4-bromo-2-methyl-5-[[(3~{R},5~{R})-1-methyl-5-phenyl-piperidin-3-yl]amino]pyridazin-3-one | C17 H21 Br N4 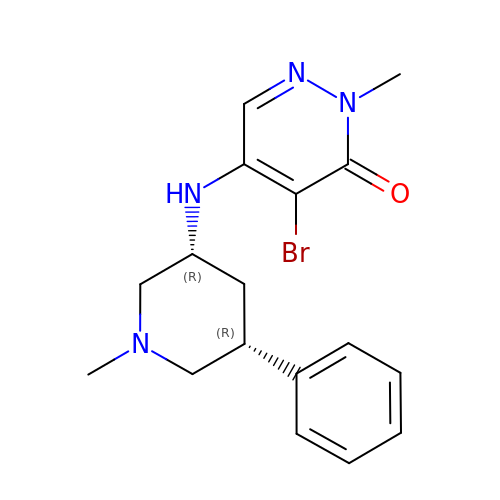O | VZAFGXCWAWRULT-UONOGXRCSA-N> EETLLE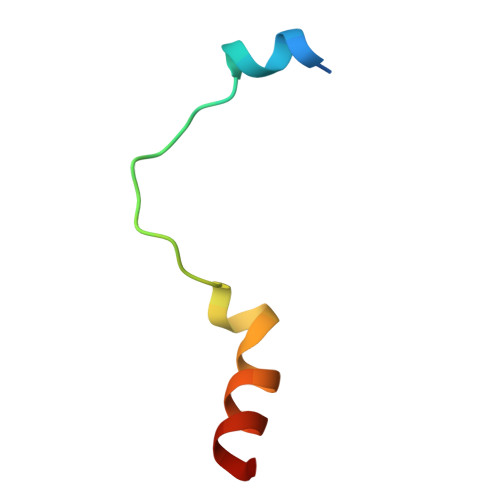LNNRIRVRKQDFTLPWEEYGELILENARKS>MSDFNLVGVIRVMPTDPDVNLDELEEKLKKVIPEKYGLAKVEREPIAFGLVALKFYVLGRDEEGYSFDEVAEKFEE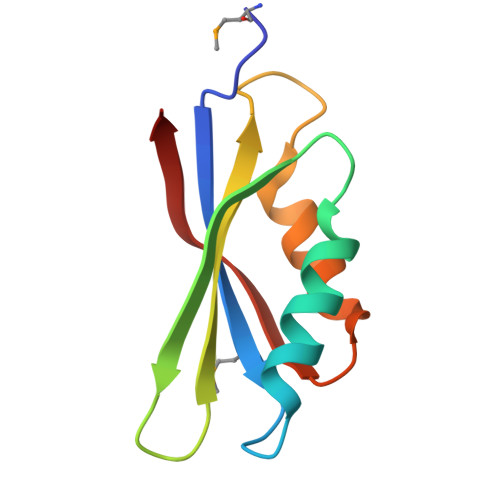VENVESAEVETVSRI[3x]> GDETKMQSLVGYVVLKDNERAILITDTKAPGKEDYNLSEGQLMNKFKNNIVIVGLSEIDNTDD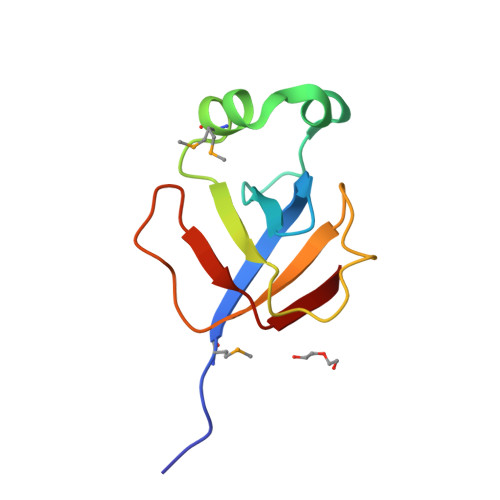LKRGEKIKVWFHTRKESNPPSATIQKYELL>MEYRYDDNATNVKAMKYLIEHYFDNFKVDSIEIIGSGYDSVAYLVNNEYIFKTKFSTNKKKGYAKEKAIYNFLNTNLETNVKIPNIEYSYISDELSILGYKEIKGTFLTPEIYSTMSEEEQNLLKRDIASFLRQMHGLDYTDISECTIDNKQNVLEEYILLRETIYNDLTDIEKDYIESFMERLNATTVFEGKKCLCHNDFSCNHLLLDGNNRLTGIIDF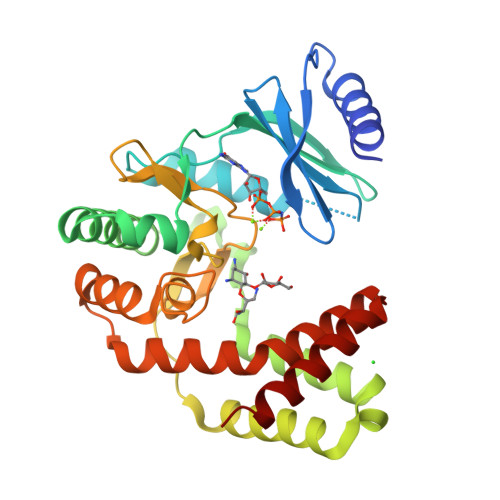GDSGIIDEYCDFIYLLEDSEEEIGTNFGEDILRMYGNIDIEKAKEYQDIVEEYYPIETIVYGIKNIKQEFIENGRKEIYKRTYKD[4x]1-[3-[[4-[(4-bromophenyl)methyl]piperazin-1-yl]methyl]phenyl]azetidin-2-one | 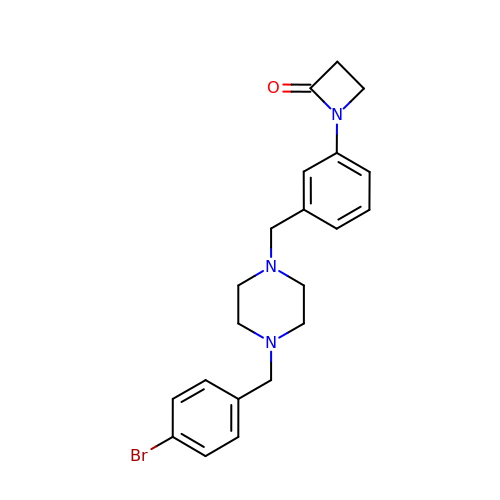C21 H24 Br N3 O | UKZMZNGKMQQUCK-UHFFFAOYSA-N> LEGENSKQKVQMSIHQFTNICFKKCVESVNDSNLSSQEEQCLSNCVNR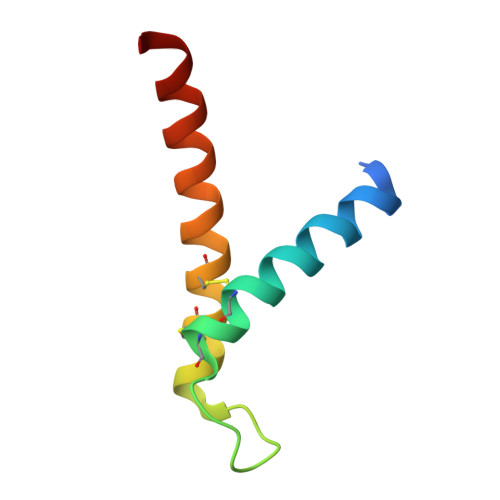FLDTNIRIVNGLQNTR> MVPAESNAVQAKLAKTLQRFENKIKAGDYYEAHQTLRTIANRYVRSKSYEHAIELISQGALSFLKAKQGGSGTDLIFYLLEVYDLAEVKVDDISVARLVRLIAELDPSEPNLKDVITGMNNWSI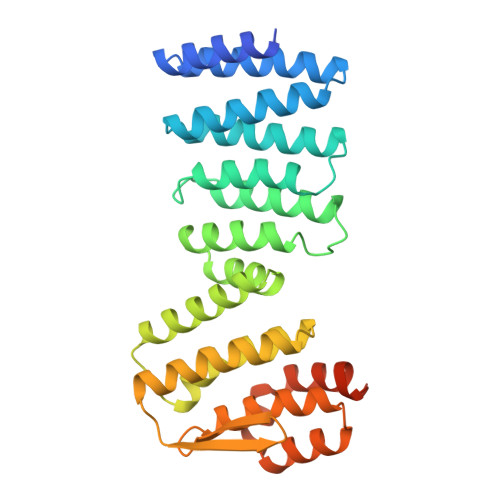KFSEYKFGDPYLHNTIGSKLLEGDFVYEAERYFMLGTHDSMIKYVDLLWDWLCQVDDIEDSTVAEFFSRLVFNYLFISNISFAHESKDIFLERFIEKFHPKYEKIDKNGYEIVFFEDYSDLNFLQLLLITCQTKDKSYFLNLKNHYLDFSQAYKSELEFLGQEYFNIVAPKQTNFLQDMMSGFLGGSK>[2x]DAFYKREMFDPAEKYKMDHRRRGIALIFNHERFFWHLTLPERRGTCADRDNLTRRFSDLGFEVKCFNDLKAEELLLKIHEVSTVSHADADCFVCVFLSHGEGNHIYA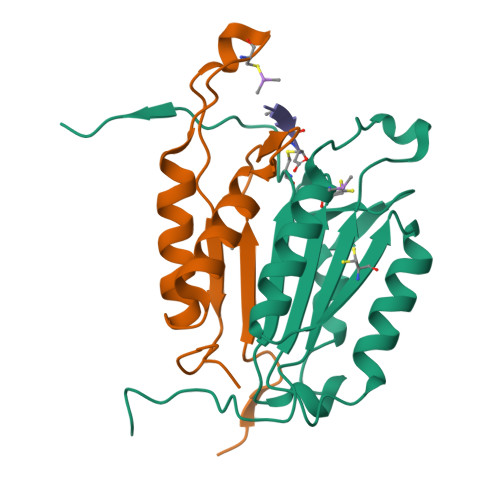YDAKIEIQTLTGLFKGDKCHSLVGKPKIFIIQACRGNQHDVPVIPLDVVD;>[2x]DAASVYTLPAGADFLMCYSVAEGYYSHRETVNGSWYIQDLCEMLGKYGSSLEFTELLTLVNRKVSQRRVDFCKDPSAIGKKQVPCFASMLTKKLHFFPKSNRHHHHHH>GGPQIFFSMGNSATISAPEHSLADAVTAWFPENKQSDVSQIWHAFEHEEHANTFSAFLDRLSDTVSARNTSGFREQVAAWLEKLSASAELRQQSFAVAADATESCEDR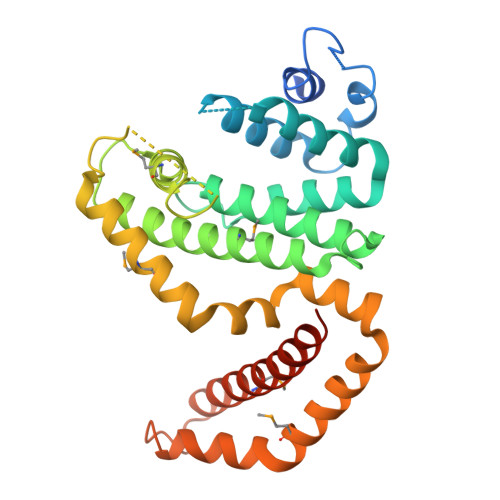VALTWNNLRKTLLVHQASEGLFDNDTGALLSLGREMFRLEILEDIARDKVRTLHFVDEIEVYLAFQTMLAEKLQLSTAVKEMRFYGVSGVTANDLRTAEAMVRSREENEFTDWFSLWGPWHAVLKRTEADRWAQAEEQKYEMLENEYSQRVADRLKASGLSGDADAEREAGAQVMRETEQQIYRQLTDEVLALRLSENGSNHIA[3x]> MVNKMDIIPEITRKSITDLINNKERIDGRSLHEFRDISIETGVISKAEGSSRVKLGNTQIIVGVKPQIGEPFPDTPEMGVILTNSELLPMASPTFEPGPPDERSVELSRVVDRCIRESRMIDLEKLCIIEGSKVWMLFLDLHIIDYDGNLFDAAVLATVAALLDTRIPAAEVEDGEVVINREKMQP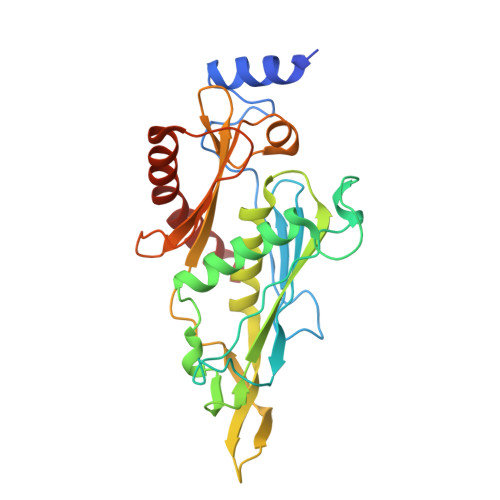LPVNRKALMCTFAKIGNEIVLDPSLEEEDILTARISIGVTEEGSICAMQKGGEGPLTRDDVLKAVSIAVEKVPQLIEYLDKSMTP> MNINATLIGQSVAFFIFVLFCMKFVWPPVIAALQERQKKIADGLDAANRA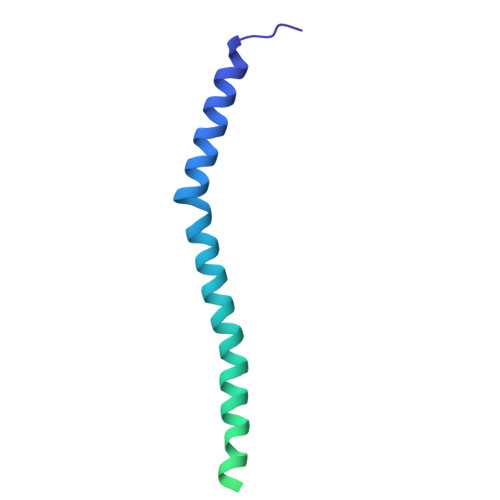ARDLELAHEKAGQQLREAKAQAAEIVEQAKKRANQIVDEARDQARTEGERLKAQAQAEIEQELNSVKDALRAQVGALAVTGAEKILGASIDANAHEQLVSKLAAEI> MNNGSGRYLLTPPDDLHPYVPSSKPQEQVYPDFKPWEHTAAEDQILANFVAKGFYHTPMVNFESISARSSVHESLVTQSNILSQQFDKIIKIREDHINKIPSNSTTTLHGPGFQLPNRITLTDHRKETWLHELSSSHTSLVKIGKFIPHGLKRRQVIEQCYLKFIPLKRAIWLIKCCYFIEWKSNHKKKRSNAAGADDAISMHLLKDWTDTFVYILEKLIFDMTNHYNDSQQLRTWKRQISYFLKLLGNCYSLRLINKEIFHHWLVEFINKMENFEFLPLSLHILMIFWNDICQIDTNAPVAATITSSQKEPFFLVTKITDMLLHKYYIVSSSKSMINDENYIINDIKK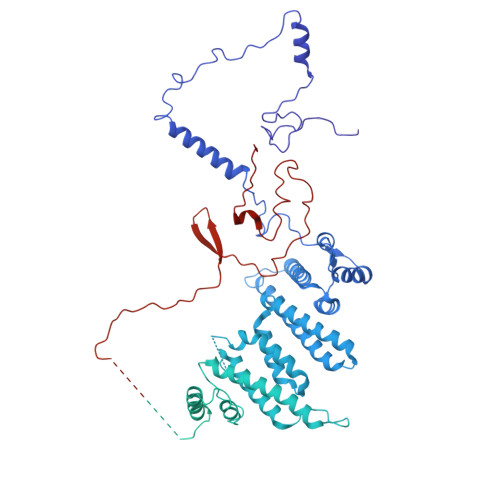NNKIKLNILKILSSLILKIFQEQSLEVFIFPTSNWEIYKPLLFEIVSNADTNQNSDMKKKLELISYRNESLKNNSSIRNVIMSASNANDFQLTIVTCKQFPKLSCIQLNCIDTQFTKLLDDNPTEFDWPTYVDQNPLTMHKIIQLILWSIHPSRQFDHYESNQLVAKLLLLRINSTDEDLHEFQIEDAIWSLVFQLAKNFSAQKRVVSYMMPSLYRLLNILITYGIIKVPTYIRKLISSGLLYLQDSNDKFVHVQLLINLKISPLMKSQYNMVLRNVMEYDVKFYEIFNFDQLVEITEQIKMRILSNDITNLQLSKTPLSIKIMVAEWYLSHLCSGILSSVNRTVLLKIFKIFCIDLEVFHHFFKWIEFIVYHQLLSDIESLEALMDILLCYQKLFSQFINDHILFTKTFIFIYKKVLKEKDVPAYNVTSFMPFWKFFMKNFPFVLKVDNDLRIELQSVYNDEKLKTEKLKNDKSEVLKVYSMINNSNQAVGQTWNFPEVFQVNIRFLLHNSEIIDTNTSKQFQKARNNVMLLIATNLKEYNKFMSIFLKRKDFTNKNLIQLISLKLLTFEVTQNVLGLEYIIRLLPINLENNDGSYGLFLKYHKEQFIKSNFEKILLTCYELEKKYHGNECEINYYEILLKILITYGSSPKLLATSTKIIMLLLNDSVENSSNILEDILYYSTCPSETDLNDIPLGSGQPDNDTVVTNDDKSDDDDHTVDEIDHVEYYVMMDFANLWVFQAFTCFCIKKIMENNEPAMAMEDLKNFIFQIIEITNSNDLCSQIFDQLKDMQTIEMITQIVEKDFCTSCLQNNNQKIDDNYIVVVIEIITSLSMRFQRETSGMIVISMENYHLLIKIIRQLSELNEGNLSKREIQIDAVLKIFSFHQDSIFQRIIADLSADKPTSPFIDSICKLFDKISFNLRLKLFLYEILSSLKSFAIYSSTIDAPAFHTSGKVELPKKLLNLPPFQVSSFVKETKLHSGDYGEEEDADQEESFSLNLGIGIVEIAHENEQKWLIYDKKDHKYVCTFSMEPYHFISNYNTKYTDDMATGSNDTTAFNDSCVNLSLFDARFERKNPH ISG15 is a ubiquitin-like protein that is activated by an E1 enzyme (Uba7) and transferred to a cognate E2 enzyme (UBE2L6) to form a UBE2L6-ISG15 intermediate that functions with E3 ligases that catalyze conjugation of ISG15 to target proteins. E1 occupies the apex of the Ub/Ubl conjugation cascade where it performs two main functions: (1) specific activation of Ub/Ubl in a two-step process that results in the formation of a thioester bond between Ub/Ubl and an E1 catalytic cysteine (adenylation and thioester bond formation) and (2) recruitment of cognate E2 enzymes followed by transfer of Ub/Ubl to an E2 catalytic cysteine (thioester transfer). While Uba1 (E1) is specific to Ub activation, ISG15 is exclusively activated by Uba7 (E1) and specifically transferred to the E2 enzyme UBE2L6. Here, we present cryo-EM structures of human Uba7 in complex with UBE2L6, ISG15 adenylate, and ISG15 thioester intermediate in a conformational state that is poised for catalysis of Uba7-UBE2L6-ISG15 thioester transfer.

The double-loaded Uba7-UBE2L6-ISG15(t)/ISG15(a) complex was prepared and imaged by single-particle cryo-electron microscopy (cryo-EM). Two reconstructions of the Uba7-UBE2L6-ISG15(t)/ISG15(a) complex were subsequently isolated, which we refer to as Form 1 and Form 2, with overall nominal resolutions of 3.38 and 3.21 Å, respectively (masked at 0.143 FSC). Both reconstructions exhibit the same overall architecture and do not appear to be functionally different, with the main difference between them being the strength of ordering of the SCCH domain, ISG15(a) NTD, and ISG15(t) CTD. Hence, we constructed a composite map and the refined coordinates derived from this map were used for descriptions of the structure below. Globally, the Uba7-UBE2L6-ISG15(t)/ISG15(a) complex exhibits a conserved architecture in both forms of the complex with the AAD, IAD, and FCCH of Uba7 engaging ISG15(a) and UBE2L6 sandwiched between the UFD and SCCH of Uba7. Consistent with the Uba7-UBE2L6-ISG15(t)/ISG15(a) complex being poised for thioester transfer, the SCCH domain of Uba7 is observed in the open conformation and the UFD adopts the proximal conformation. Density corresponding to the pyrophosphate (PPi) leaving group and Mg2+ was absent indicating that we have captured the product complex of adenylation, after PPi/Mg2+ release. While the density is modest, likely due to conformational dynamism (local resolution of 5–7 Å), the ISG15(t) CTD clearly extends away from the surface of UBE2L6 and is wedged between the UFD and SCCH domain of Uba7 (top view). Interestingly, the active site of the Uba7-UBE2L6-ISG15(t)/ISG15(a) complex represents a hybrid of the adenylation-competent open and thiolation-competent closed structures. To our surprise, ISG15(t) is located at the back of the Uba7-UBE2L6-ISG15(t)/ISG15(a) complex where it sits atop the AAD and packs against the UFD and SCCH domains.

> MDALDASKLLDEELYSRQLYVLGSPAMQRIQGARVLVSGLQGLGAEVAKNLVLMGVGSLTLHDPHPTCWSDLAAQFLLSEQDLERSRAEASQELLAQLNRAVQVVVHTGDITEDLLLDFQVVVLTAAKLEEQLKVGTLCHKHGVCFLAADTRGLVGQLFCDFGEDFTVQDPTEAEPLTAAIQHISQGSPGILTLRKGANTHYFRDGDLVTFSGIEGMVELNDCDPRSIHVREDGSLEIGDTTTFSRYLRGGAITEVKRPKTVRHKSLDTALLQPHVVAQSSQEVHHAHCLHQAFCALHKFQHLHGRPPQPWDPVDAETVVGLARDLEPLKRTEEEPLEEPLDEALVRTVALSSAGVLSPMVAMLGAVAAQEVLKAISRKFMPLDQWLYFDALDCLPEDGELLPSPEDCALRGSRYDGQIAVFGAGFQEKLRRQHYLLVGAGAIGCELLKVFALVGLGAGNSGGLTVVDMDHIERSNLSRQFLFRSQDVGRPKAEVAAAAARGLNPDLQVIPLTYPLDPTTEHIYGDNFFSRVDGVAAALDSFQARRYVAARCTHYLKPLLEAGTSGTWGSATVFMPHVTEAYRAPASAAASEDAPYPVCTVRYFPSTAEHTLQWARHEFEELFRLSAETINHHQQAHTSLADMDEPQTLTLLKPVLGVLRVRPQNWQDCVAWALGHWKLCFHYGIKQLLRHFPPNKVLEDGTPFWSGPKQCPQPLEFDTNQDTHLLYVLAAANLYAQMHGLPGSQDWTALRELLKLLPQPDPQQMAPIFASNLELASASAEFGPEQQKELNKALEVWSVGPPLKPLMFEKDDDSNFHVDFVVAAASLRCQNYGIPPVNRAQSKRIVGQIIPAIATTTAAVAGLLGLELYKVVSGPRPRSAFRHSYLHLAENYLIRYMPFAPAIQTFHHLKWTSWDRLKVPAGQPERTLESLLAHLQEQHGLRVRILLHGSALLYAAGWSPEKQAQHLPLRVTELVQQLTGQAPAPGQRVLVLELSCEGDDEDTAFPPLHYEL;>[2x]MGWDLTVKMLAGNEFQVSLSSSMSVSELKAQITQKIGVHAFQQRLAVHPSGVALQDRVPLASQGLGPGSTVLLVVDKSDEPLSILVRNNKGRSSTYEVRLTQTVAHLKQQVSGLEGVQDDLFWLTFEGKPLEDQLPLGEYGLKPLSTVFMNLRLRGG;> MASMRVVKELEDLQKKPPPYLRNLSSDDANVLVWHALLLPDQPPYHLKAFNLRISFPPEYPFKPPMIKFTTKIYHPNVDENGQICLPIISSENWKPSTKTSQVLEALNVLVNRPNIREPKRMDLADLLTQNPELFRKNAEEFTLRFGVDRPS> SGRGKGGK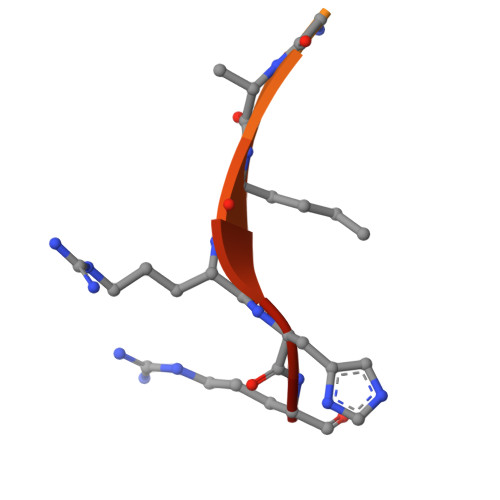GLGKGGAKRHRK>GPLGSPEFGRPGWVIGVNPDIGGAIAVLSPDGSSQVFDNPFVHI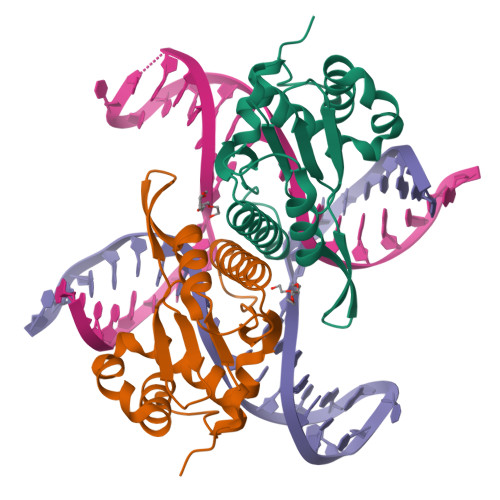VVSEVIRKRLDTKSIIQLLRGLDAPPGTTAYIEKSSPFPTDGKQGWWSTGFSYGLWIASLVASGFSVVPIASQTWKAYFGLMRSETPKDDSRQAASILFPDKDQSLKLKKHHGRAEALLLAAYGKGLVLP[2x]> MGSDKIHHHHHHENLYFQGDSFKTKSGKELTITFIKHGSLMLTYDNHSIQVDPVSEYADYTTFPKADIILITHEHGDHLDPKAIQAVEKSDTEIIANENSQKKLGKGKVLKNGDTDTSISYMKIEAVPAYNTTPGRDK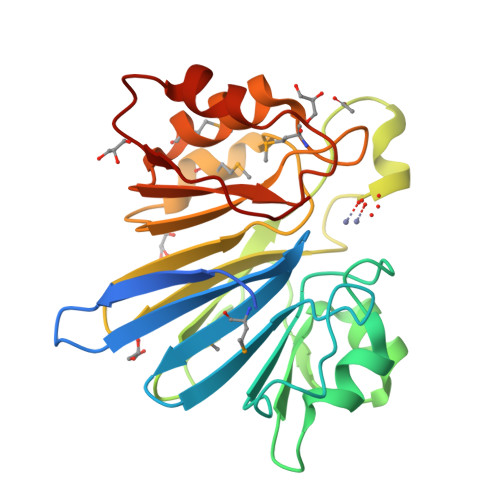YHPRHRDNGYILTFDGLRVYIAGDTEDIPEMKDLKDIDIAFLPVNQPYTMTVSQAAKAARMFSPKILYPYHYGDTKIGELKDALKDSGIDVRIRELQ> MPKSTYFSLSDEKRNRVYDACLNEFQTHSFHEAKI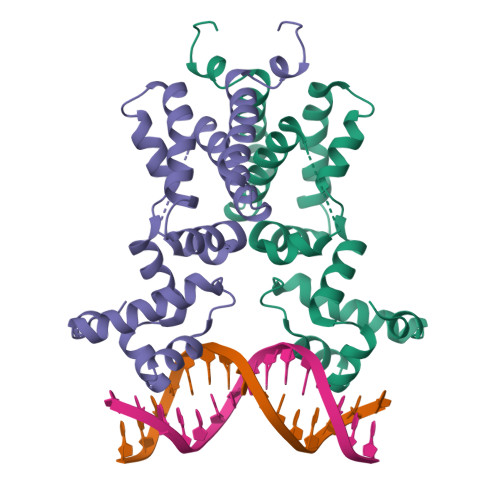MHIVKALDIPRGSFYQYFEDLKDAYFYVLSQETLEIHDLFFNLLKDNSIEESLDKYKYLLLENLIDSPQYKLYKYRFLDWTYELERDWKPQSSATVPASENDNPISQVLKSVVHNLVYRLFSENWTEKTFIENYDKEIKLVTEGLLNYITDRKN>STAGKVIKCKAAVLWELKKPFSIEEVEVAPPKAHEVRIKMVAAGICRSDEHVVSGNLVTPLPVILGHEAAGIVESVGEGVTTVKPGDKVIPLFTPQCGKCRICKNPESNYCLKNDLGNPRGTLQDGTRRFTCSGKPIHHFVGVSTFSQYTVVDENAVAKIDAASPLEKVCLIGCGFSTGYGSAVKVAKVTPGSTCAVFGLGGVGLSVVMGCKAAGAARIIAVDINKDKFAKAKELGATECINPQDYKKPIQEVLKEMTDGGVDFSFEVIGQLDTMMASLLCCHEACGTSVIVGVPPDSQN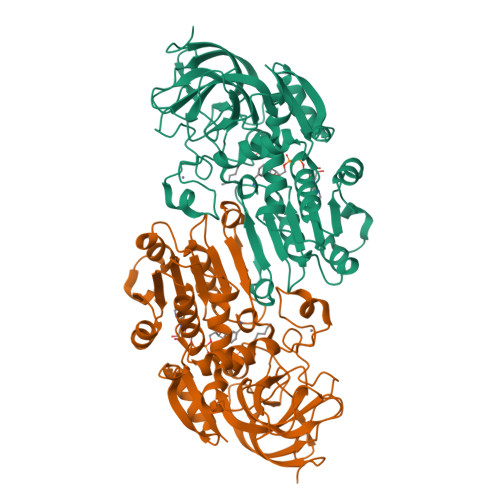LSINPMLLLTGRTWKGAIFGGFKSKESVPKLVADFMAKKFSLDALITNVLPFEKINEGFDLLRSGKSIRTVLTF[2x]>[2x]GPGSMTDFYSLIPSAPKGRFDGIERAHTAEDVKRLRGSVEIKYSLAEMGANRLWKLIHEEDFVNALGALSGNQAMQMVRAGLKAIYLSGWQVAADANTASAMY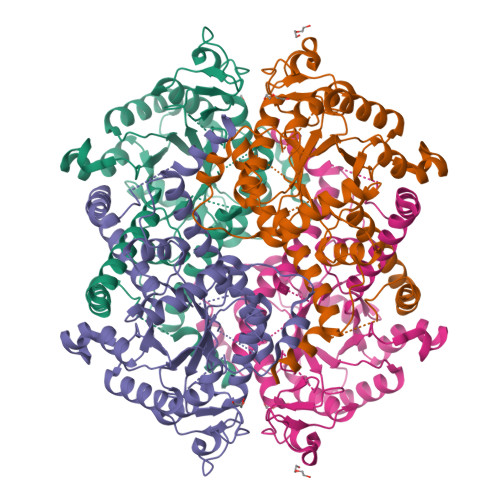PDQSLYPANAGPELAKRINRTLQRADQIETAEGKGLSVDTWFAPIVADAEAGFGDPLDAFEIMKAYIEAGAAGVHFEDQLASEKKCGHLGGKVLIPTAAHIRNLNAARLAADVMGTPTLIVARTDAEAAKLLTSDIDERDQPFVDYEAGRTAEGFYQVKNGIEPCIARAIAYAPYCDLIWMETSKPDLAQARRFAEAVHKAHPGKLLAYNCSPSFNWKKNLDDATIAKFQRELGAMGYKFQFITLAGFHQLNYGMFELARGYKDRQMAAYSELQQAEFAAEADGYTATKHQREVGTGYFDAVSLAITGGQSSTTAMKESTETAQFKPAAE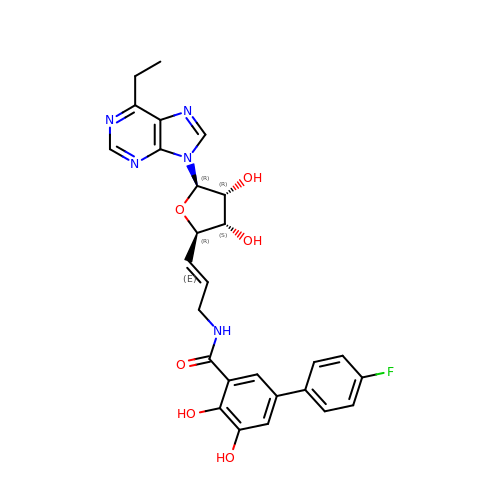~{N}-[(~{E})-3-[(2~{R},3~{S},4~{R},5~{R})-5-(6-ethylpurin-9-yl)-3,4-bis(oxidanyl)oxolan-2-yl]prop-2-enyl]-5-(4-fluorophenyl)-2,3-bis(oxidanyl)benzamide | C27 H26 F N5 O6 | XTRPLJQALBTCJE-ZYNJZHFOSA-N>TAILVTTRDGTRTEIQAEPGLSLMEALRDAGIDELLALCGGCCSCATCHVLVAPAFADRLPALSGDENDLLDSSDHRTPHSRLSCQITINDKLE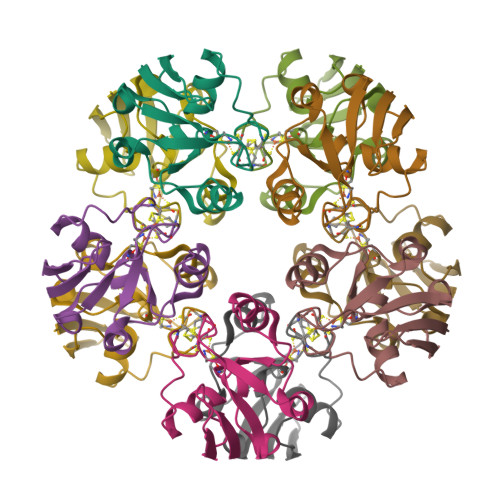GLEVEIAPED[5x]>MLGLKTSIIGRRVIYFQEITSTNEFAKTSYLEEGTVIVADKQTMGHGRLNRKWESPEGGLWLSIVLSPKVPQKDLPKIVFLGAVGVVETLKEFSIDGRIKWPNDVLVNYKKIAGVLVEGKGDKIVLGIGLNVNNKVPNGATSMKLELGSEVPLLSVFRSLITNLDRLYLNFLKNPMDILNLVRDNMILGVRVKILGDGSFEGIAEDIDDFGRLIIRLDSGEVKKVIYGDVSLRFL[2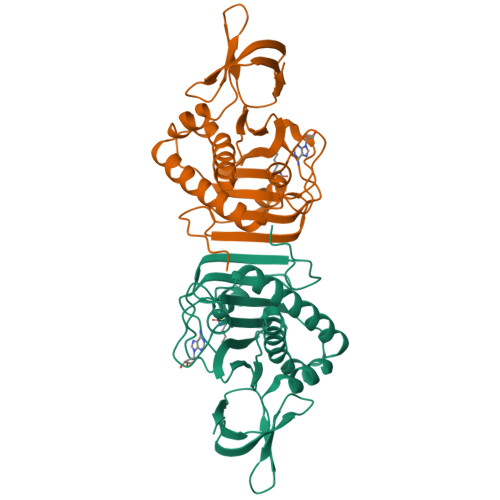x]> ETVLADRFERLVELVTMMGDQGELPIAMALANVVPCSQWDELARVLVTLFDSRHLLYQLLWNMFSKEVELADSMQTLFRGNSLASKIMTFCFKVYGATYLQKLLDPLLRIVITSSDWQHVSFEVDPTRLEPSESLEENQRNLLQMTEKFFHAIISSSSEFPPQLRSVCHCLYQVVSQRFPQNSIGAVGSAM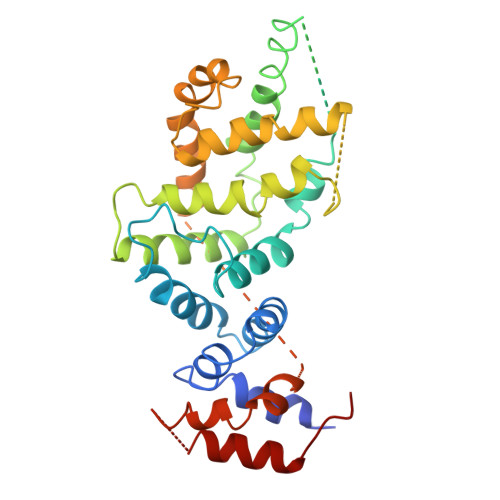FLRFINPAIVSPYEAGILDKKPPPIIERGLKLMSKILQSIANHVLFTKEEHMRPFNDFVKSNFDAARRFFLDIASDCPTSDAVNHSLSFISDGNVLALHRLLWNNQEKIGQYLSSNRDHKAVGRRPFDKMATLLAYLGPPEH To make further progress, we present here a first characterization of a novel tetrameric ion channel, referred to as NaKTs, with an unusual proline-rich selectivity filter sequence using X-ray crystallography, electrophysiology and MD simulations. Single-channel recordings demonstrate that the NaKTs channel is a Ca2+-activated non-selective cation channel. The NaKTs channel belongs to the family of channels with fourfold symmetric tetrameric pore domains. The X-ray structures revealed the presence of Ca2+ binding sites, SCa, formed by main chain atoms of residues Pro63, Gly65, Ser59 and Leu62, near the intracellular end of the selectivity filter.

Three different diffraction datasets were analyzed to identify different ion occupancy states (by virtue of the I4 space group symmetry, the six monomers yield three crystallographically related tetramers). A total of nine crystallographically distinct tetramers were considered in the analysis, revealing four different occupancy states, I to IV, with 0, 2, 3 and 6 Ca2+ ions, respectively. In state IV, there are four Ca2+ ions in SCa and two additional Ca2+ ions, one in the site corresponding to S3 in KcsA near Gly65 and a second ion near Pro63 (a different sub-state is seen with the ion position shifted by 2.1 and 1.1 Å towards the intracellular surface). Lastly, there is a tetramer with a single Ca2+ ion located at the centre of the intracellular vestibule with no ions observed in the pore, as observed in the KcsA and NaK structures, assigned to State I. More details about the locations of Ca2+ ions in the 3.4 Å dataset 3 (3.4 Å resolution) and 3.6 Å dataset 1 (3.6 Å resolution) crystal structures are provided in Supplementary Fig. 5. Analysis of crystallographic data indicates that the presence of bound Ca2+ at diagonally-opposing sites inside the selectivity filter controls the diameter of the conducting pore.

>[6x]MLGLTLMFKRFFGAVRTSWRDPSTRGAVLSLAIIVTAATIFYTLAEKWSVIDSLFYAVSVGLPMGNGPLSPTLTLSKIFTLVYAILVVGLFVTVGGSLASAIVQNNTEKFKRLNRKGSAEAEDHHHHHH> MVDMSKVKLRIENIVASVDLFAQLDLEKVLDLCPNSKYNPEEFPGIICHLDDPKVALLIFSSGKLVVTGAKSVQDIERAVAKLAQKLKSIGVKFKRAPQIDVQNMVFSGDIGREFNLDVVALTLPNCEYEPEQFPGVIYRVKEPKSVILLFSSGKIVCSGAKSEADAWEAVRKLLRELDKYL;> VSDAAERNLAFALSELDRITAQLKLPRHVEEEAARLYREAVRKGLIRGRS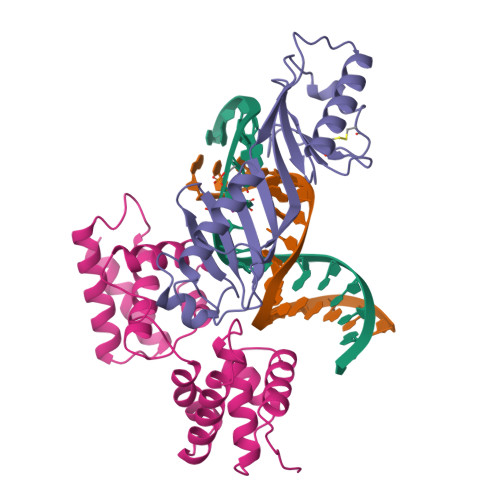IESVMAACVYAACRLLKVPRTLDEIADIARVDKKEIGRSYRFIARNLNLTPKKLFVKPTDYVNKFADELGLSEKVRRRAIEILDEAYKRGLTSGKSPAGLVAAALYIASLLEGEKRTQREVAEVARVTEVTVRNRYKELVEKLKIKVPIA3-(2-chlorophenyl)-4~{H}-1,2,4-triazole | C8 H6 Cl N3 | 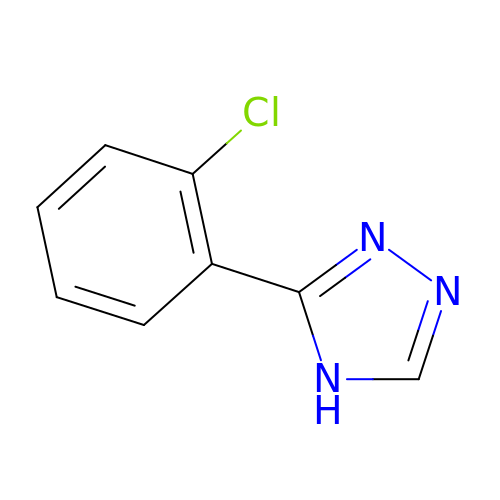HUJUBANPLITKPV-UHFFFAOYSA-N> MRGSHHHHHHGIRMTRISREMMKELLSVYFIMGSNNTKADPVTVVQKALKGGATLYQFREKGGDALTGEARIKFAEKAQAACREAGVPFIVNDDVELALNLKADGIHIGQEDANAKEVRAAIGDMILGVSAHTMSEVKQAEEDGADYVGLGPIYPTETAKDTRAVQGVSLIEAVRRQGISIPIVGIGGITIDNAAPVIQA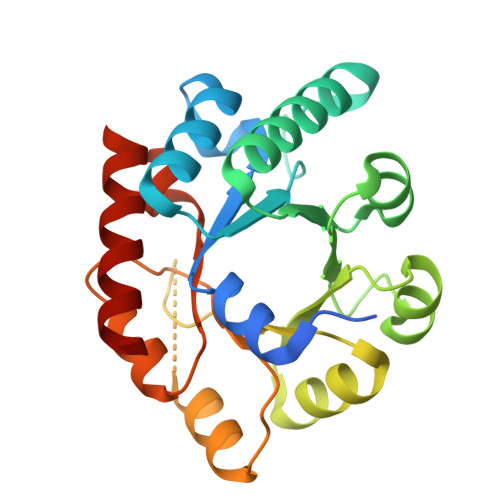GADGVSMISAISQAEDPESAARKFREEIQTYKTGR>[2x]MATKGGTVKAASGFNAMEDAQTLRKAMKGLGTDEDAIISVLAYRNTAQRQEI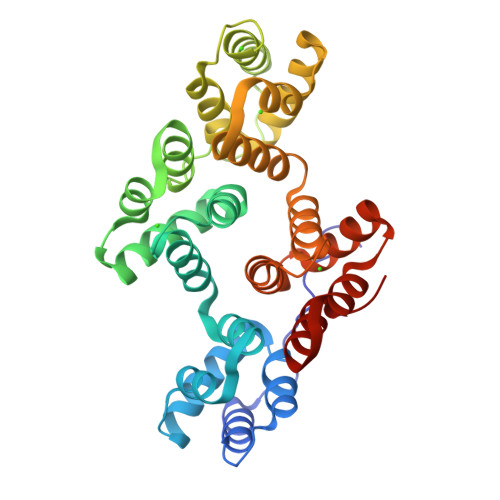RTAYKSTIGRDLIDDLKSELSGNFEQVIVGMMTPTVLYDVQELRRAMKGAGTDEGCLIEILASRTPEEIRRISQTYQQQYGRSLEDDIRSDTSFMFQRVLVSLSAGGRDEGNYLDDALVRQDAQDLYEAGEKKWGTDEVKFLTVLCSRNRNHLLHVFDEYKRISQKDIEQSIKSETSGSFEDALLAIVKCMRNKSAYFAEKLYKSMKGLGTDDNTLIRVMVSRAEIDMLDIRAHFKRLYGKSLYSFIKGDTSGDYRKVLLVLCGGDD>[2x]MKLYVFLVNTGTTLTFDTELTVQTVADLKHAIQSKYKIAIQHQVLVVNGGECMAADRRVCTYSAGTD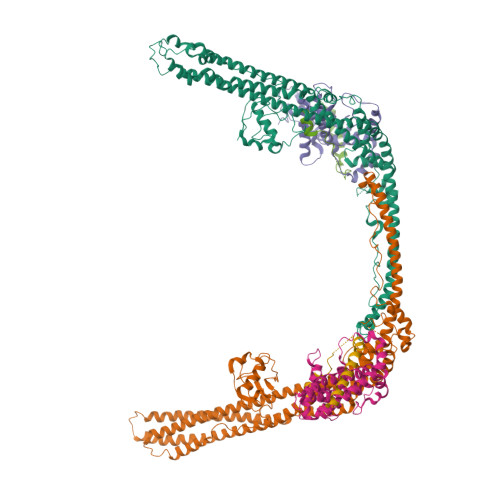TNPIFLFNKEMILCDRPPAIPKTTFSTENDMEIKVEESLMMPAVFHTVASRTQLALEMYEVAKKLCSFCEGLVHDEHLQHQGWAAIMANLEDCSNSYQKLLFKFESIYSNYLQSIEDIKLKLTHLGTAVSVMAKIPLLECLTRHSYRECLGRLDSLPEHEDSEKAEMKRSTELVLSPDMPRTTNESLLTSFPKSVEHVSPDTADAESGKEIRESCQSTVHQQDETTIDTKDGDLPFFNVSLLDWINVQDRPNDVESLVRKCFDSMSRLDPRIIRPFIAECRQTIAKLDNQNMKAIKGLEDRLYALDQMIASCGRLVNEQKELAQGFLANQKRAENLKDASVLPDLCLSHANQLMIMLQNHRKLLDIKQKCTTAKQELANNLHVRLKWCCFVMLHADQDGEKLQALLRLVIELLERVKIVEALSTVPQMYCLAVVEVVRRKMFIKHYREWAGALVKDGKRLYEAEKSKRESFGKLFRKSFLRNRLFRGLDSWPPSFCTQKPRKFDCELPDISLKDLQFLQSFCPSEVQPFLRVPLLCDFEPLHQHVLALHNLVKAAQSLDEMSQTITDLLSEQK;>MEQEHTEILRGLRFTLLFVQHVLEIAALKGSASEAAGGPEYQLQESVVADQISLLSREWGFAEQLVLYLKVAELLSSGLQSAIDQIRAGKLCLSSTVKQVVRRLNELYKASVVSCQGLSLRLQRFFLDKQRLLDRIHSITAERLIFSHAVQMVQSAALDEMFQHREGCVPRYHKALLLLEGLQHMLSDQADIENVTKCKLCIERRLSALLTGICA[2x];>[2x]HDVLETIFVRKVGAFVNKPINQVTLTSLDIPFAMFAPKNLELEDTDPMVNPPDSPETESPLQGSLHSDGSSGGSSGNTHDDFVMIDFKPAFSKDDILPMDLGTFYREFQNPPQLSSLSIDIGAQSMAEDLDSLPEKLAVHEKNVREFDAFVETLQ>[8x]SLTTQRLGLIMNGVTGRMGLNQHLIRSIVAIRDQGGVRLKNGDRIMPDPILVGRSAEKVEALAKRFNIARWTTDLDAALADKNDTMFFDAATTQARPGLLTQAINAGKHVYCEKPIATNFEEALEVVKLANSKGVKHGT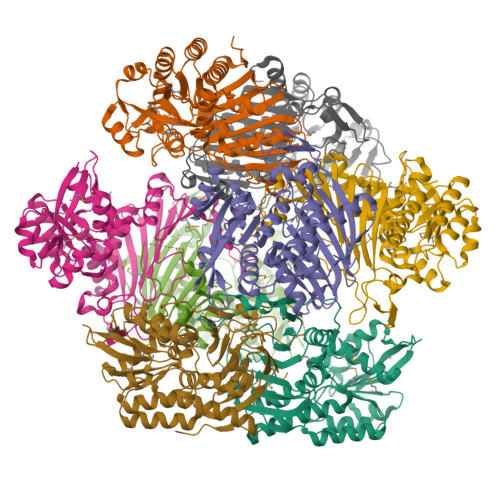VQDKLFLPGLKKIAFLRDSGFFGRILSVRGEFGYWVFEGGWQEAQRPSWNYRDEDGGGIILDMVCHWRYVLDNLFGNVQSVVCIGNTDIPERFDEQGKKYKATADDSAYATFQLEGGVIAHINMSWVTRVYRDDLVTFQVDGTHGSAVAGLSDCMIQARQATPRPVWNPDEKRLHDFYGDWQKLPDNVSYDNGFKEQWEMFIRHVYEDAPYKFTLLEGAKGVQLAECALKSWKERRWIDVAPIK> PFVEDWDLVQTLGEGAYGEVQLAVNRVTEEAVAVKIVDMKRAVDCPENIKKEICILKMLNHENVIKFYGHRREGNIQYLFMELASGGSLFDRIEPDIGMPEPDAQRFFHQLMAG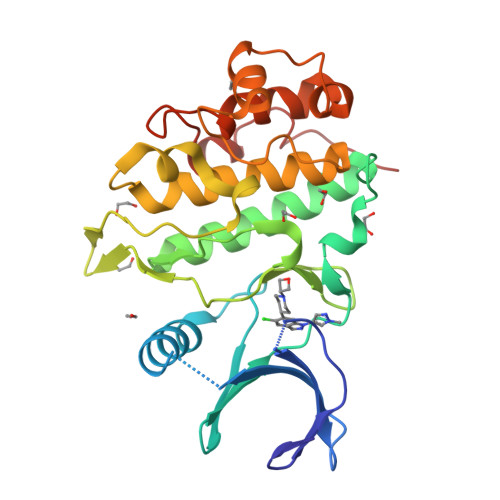VVYLHGIGITHRDIKPHNLLLDERDNLKIADYSLATVFRYNNRERLLNKMCGTLPYVAPELLKRREFHAEPVDVWSCGIVLTAMLAGELPWDQPSDSCQEYSDWKEKKTYLNPWKKIDSAPLALLHKILVENPSARITIPDIKKDRWYNKPLKK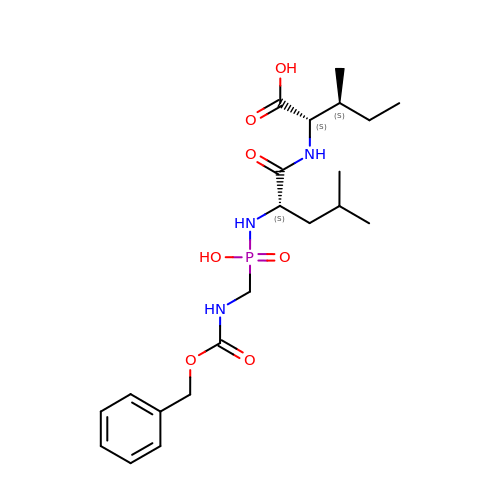N-[(S)-({[(benzyloxy)carbonyl]amino}methyl)(hydroxy)phosphoryl]-L-leucyl-L-isoleucine | C21 H34 N3 O7 P | WXJWRPSIWAFMIG-SZMVWBNQSA-N> MPQTVVEADISREPDDVPPPIGKRAPQTVRVDLLSVELEGRLAEGTTFGYWTFNGKVPGPLLRVRVGDTVEIHLKNAADSAMIHSVDFHAAIAPGGGAAALQVEPGGEKAITWKALVPGLFVYHCATPMV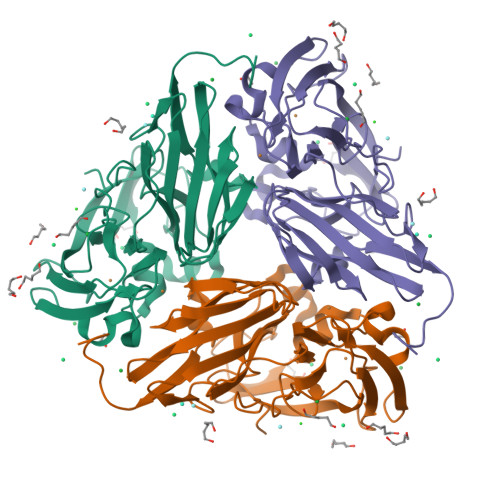AEHIANGMYGMILVEPEGGLPPVDHEFYVMQGEIYSDIPYGQHGSAEFSVEKLLAERPEYFVFNGSVGALSKLHPLKAKVGDTVRIFFGVGGPNHASSFHVIGEIFDKVDLFGGLTTPPLAGIQTVTVPPGGAAIAEFKVEVPGTYTLVDHALARAERGLLGILHVQGPENPDIYNGVALPGAGHENLYFQ>[4x]GTAGKVIKCKAAVLWEQKQPFSIEEIEVAPPKTKEVRIKILATGICRTDDHVIKGTMVSKFPVIVGHEATGIVESIGEGVTTVKPGDKVIPLFLPQCRECNACRNPDGNLCIRSDITGRGVLADGTTRFTC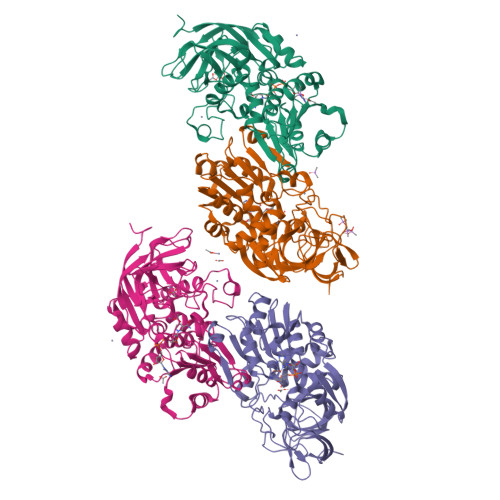KGKPVHHFLNTSTFTEYTVVDESSVAKIDDAAPPEKVCLIGCGFSTGYGAAVKTGKVKPGSTCVVFGLGGVGLSVIMGCKSAGASRIIGIDLNKDKFEKAMAVGATECISPKDSTKPISEVLSEMTGNNVGYTFEVIGHLETMIDALASCHMNYGTSVVVGVPPSAKMLTYDPMLLFTGRTWKGCVFGGLKSRDDVPKLVTEFLAKKFDLDQLITHVLPFKKISEGFELLNSGQSIRTVLTF Next, a β-keto acid cleavage enzyme (BKACE)28,29 converts the non-native substrate MSA with acetyl-CoA into acetoacetate and formyl-CoA. The Claisen-like condensation reaction accepts various β-keto acids that react with acetyl-CoA to form an acyl-CoA ester and acetoacetate. In these assays, BKACE15 from Paracoccus denitrificans performed best. BKACE15 forms a homotetramer where each active site is accommodated in a TIM-barrel fold, and consists of eight β-sheets that are surrounded by eight α-helices.

Each active site also exhibits only one entry channel for both substrates that appears fully occupied upon acetyl-CoA binding. The surface representation of acetyl-CoA highlights the complete occupancy of the entry channel. After the reaction has taken place, formyl-CoA is released before acetoacetate can leave the active site. This hypothesis is further corroborated by the observation that acetoacetate is an inhibitor for the reaction with MSA and acetyl-CoA. However, we also observed that the enzyme was inhibited by its product acetoacetate with a half-maximal inhibitory concentration (IC50) of 1.45 ± 0.16 mM. Substrate labeling is shown in yellow for acetyl-CoA (“ACO”) and acetoacetate (“AAE”) and in dark grey for CoA (“COA”) and malonate (“MLI”). Earlier studies had proposed R254 as a catalytic base involved in the reaction. However, our structures with bound CoA-ester prompted us to revisit the nature of the catalytic base and suggest a different mechanism for the reaction with MSA, in which E171 acts as the catalytic base (discussed in more detail in Supplementary Note 2). Replacing E171 by leucine abolished BKACE activity, while substitution by a chemically similar but shorter aspartate still showed basal activity (5% of the wild type), supporting the role of E171 in catalysis.

>[2x]MGHHHHHHHHHHSSGHIEGRHGSRMSLNGKVIITCAVTGAIHTPSMSPYLPVSASEITDAAIGAAEAGAAVIHLHARHEGDGSPDQSVEAFNPILGVIKQASDAVLNITTGGAPTMSIAERIQPAQHYRPELASLNMGTMNFGLFPMLNRYESQLKHQWERNYLGNKDIIFRNTFGDVEHVMTTLGAGGTRFEFECYDTSHLYNLKHFYDRGLVKGPLFIQTVFGLMGGIGAHPDDVLHMKRTADRLFGQDYRWSVLGAGRNQLNIAAMSAAMGGHVRVGLEDNLWAGKGRLAETNAQQVRAARQIVEGLGLEVATPAEARELLALKGGDQVNF> MGSADAQSFLNRVCGVSAARLTPCGTGTSTDVVYRAFDIYNDKVAGFAKFLKTNCCRFQEKDEDDNLIDSYFVVKR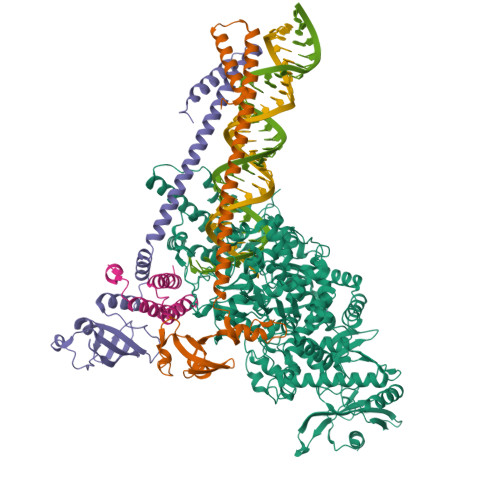HTFSNYQHEETIYNLLKDCPAVAKHDFFKFRIDGDMVPHISRQRLTKYTMADLVYALRHFDEGNCDTLKEILVTYNCCDDDYFNKKDWYDFVENPDILRVYANLGERVRQALLKTVQFCDAMRNAGIVGVLTLDNQDLNGNWYDFGDFIQTTPGSGVPVVDSYYSLLMPILTLTRALTAESHVDTDLTKPYIKWDLLKYDFTEERLKLFDRYFKYWDQTYHPNCVNCLDDRCILHCANFNVLFSTVFPPTSFGPLVRKIFVDGVPFVVSTGYHFRELGVVHNQDVNLHSSRLSFKELLVYAADPAMHAASGNLLLDKRTTCFSVAALTNNVAFQTVKPGNFNKDFYDFAVSKGFFKEGSSVELKHFFFAQDGNAAISDYDYYRYNLPTMCDIRQLLFVVEVVDKYFDCYDGGCINANQVIVNNLDKSAGFPFNKWGKARLYYDSMSYEDQDALFAYTKRNVIPTITQMNLKYAISAKNRARTVAGVSICSTMTNRQFHQKLLKSIAATRGATVVIGTSKFYGGWHNMLKTVYSDVENPHLMGWDYPKCDRAMPNMLRIMASLVLARKHTTCCSLSHRFYRLANECAQVLSEMVMCGGSLYVKPGGTSSGDATTAYANSVFNICQAVTANVNALLSTDGNKIADKYVRNLQHRLYECLYRNRDVDTDFVNEFYAYLRKHFSMMILSDDAVVCFNSTYASQGLVASIKNFKSVLYYQNNVFMSEAKCWTETDLTKGPHEFCSQHTMLVKQGDDYVYLPYPDPSRILGAGCFVDDIVKTDGTLMIERFVSLAIDAYPLTKHPNQEYADVFHLYLQYIRKLHDELTGHMLDMYSVMLTNDNTSRYWEPEFYEAMYTPHTVLQHHHHHHHHHH;>GPAIASEFSSLPSYAAFATAQEAYEQAVANGDSEVVLKKLKKSLNVAKSEFDRDAAMQRKLEKMADQAMTQMYKQARSEDKRAKVTSAMQTMLFTMLRKLDNDALNNIINNARDGCVPLNIIPLTTAAKLMVVIPDYNTYKNTCDGTTFTYASALWEIQQVVDADSKIVQLSEISMDNSPNLAWPLIVTALRANSAVKLQ[2x];> GPSKMSDVKCTSVVLLSVLQQLRVESSSKLWAQCVQLHNDILLAKDTTEAFEKMVSLLSVLLSMQGAVDINKLCEEMLDNRATLQ> VAERDSVMLGEIAPHH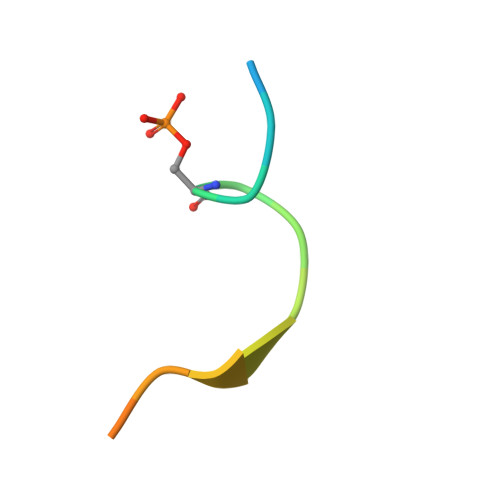DY>[5x]MKAHPKEMVPLMGKRVAAPSGNPAILPEKRPAEI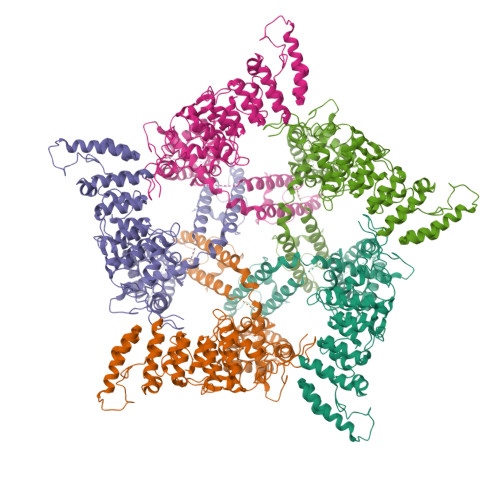TPTKKSAHFFLEIEGFEPNPTVAKTSPPVFSKPMDSNIRQCISGNCDDMDSPQSPQDDVTETPSNPNSPSAQLAKEEQRRKKRRLKKRIFAAVSEGCVEELVELLVELQELCRRRHDEDVPDFLMHKLTASDTGKTCLMKALLNINPNTKEIVRILLAFAEENDILGRFINAEYTEEAYEGQTALNIAIERRQGDIAALLIAAGADVNAHAKGAFFNPKYQHEGFYFGETPLALAACTNQPEIVQLLMEHEQTDITSRDSRGNNILHALVTVAEDFKTQNDFVKRMYDMILLRSGNWELETTRNNDGLTPLQLAAKMGKAEILKYILSREIKEKRLRSLSRKFTDWAYGPVSSSLYDLTNVDTTTDNSVLEITVYNTNIDNRHEMLTLEPLHTLLHMKWKKFAKHMFFLSFCFYFFYNITLTLVSYYRPREEEAIPHPLALTHKMGWLQLLGRMFVLIWAMCISVKEGIAIFLLRPSDLQSILSDAWFHFVFFIQAVLVILSVFLYLFAYKEYLACLVLAMALGWANMLYYTRGFQSMGMYSVMIQKVILHDVLKFLFVYIVFLLGFGVALASLIEKCPKDNKDCSSYGSFSDAVLELFKLTIGLGDLNIQQNSKYPILFLFLLITYVILTFVLLLNMLIALMGETVENVSKESERIWRLQRARTILEFEKMLPEWLRSRFRMGELCKVAEDDFRLCLRINEVKWTEWKTHVSFLNEDPGPVRRTDFNKIQDSSRNNSKTTLNAFEEVEEFPETSV> LRAGMQKLACGKLTGISDPVTVKTSGSRFGSWMTDPLAPEGDNRVWYMDGYHNNRFVREYKSMVDFMNTDNFTSHRLPHPWSGTGQVVYNGSIYFNKFQSHIIIRFDLKTETILKTRSLDYAGYNNMYHYAWGGHSDIDLMVDESGLWAVYATNQNAGNIVVSRLDPVSLQTLQTWNTSYPKRSAGEAFIICGTLYVTN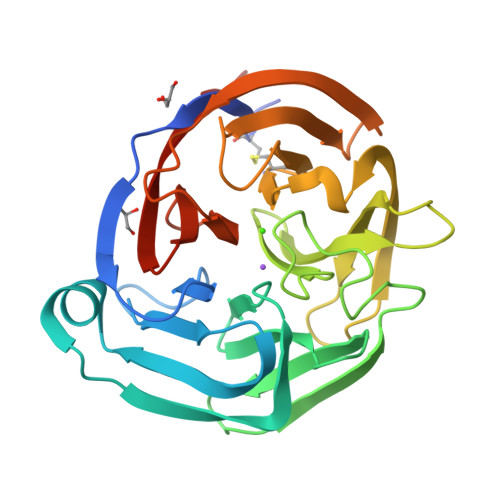GYSGGTKVHYAYQTNASTYEYIDIPFQNKYSHISMLDYNPKDRALYAWNNGHQILYNVTLFHVIRSDEL> MANKQQNFNTGIKDFDFWLSEVEALLASEDYGKDLASVNNLLKKHQLLEADISAHEDRLKDLNSQADSLMTSSAFDTSQVKDKRETINGRFQRIKSMAA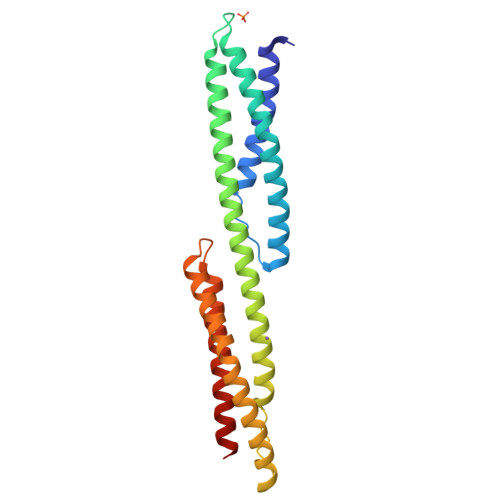ARRAKLNESHRLHQFFRDMDDEESWIKEKKLLVSSEDYGRDLTGVQNLRKKHKRLEAELAAHEPAIQGVLDTGKKLSDDNTIGKEEIQQRLAQFVDHWKELKQLAAARGQRLEESLE(2S,3S,4S,5R)-2-{[(4-methylpentyl)sulfonyl]methyl}piperidine-3,4,5-triol | C12 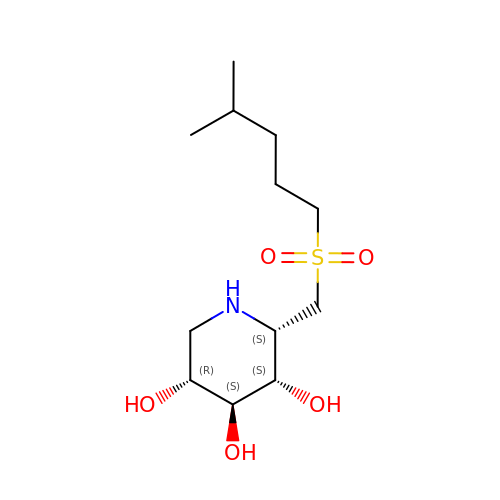H25 N O5 S | MIGRFAIIVQTLPR-WYUUTHIRSA-N Leucine Rich Repeat Kinase 1 and 2 (LRRK1 and LRRK2) are homologs in the ROCO family of proteins in humans. LRRK1 and LRRK2 have a similar domain organization: an N-terminal half containing Ankyrin (ANK) and Leucine Rich Repeats (LRR), and a catalytic C-terminal half containing the ROC–COR ROCO signature, followed by the kinase and a WD40 domain. Despite their shared domain architecture and involvement in intracellular trafficking, their disease associations are strikingly different: LRRK2 is involved in familial Parkinson’s disease while LRRK1 is linked to bone diseases. LRRK1 and LRRK2 use different mechanisms of autoinhibition, with LRRK1 having a second level of autoinhibition absent in LRRK2.

We purified LRRK1(Δ1–19), where the N-terminal 19 residues, predicted to be disordered, were deleted, and imaged it in the presence of Rab7a, ATP and GTP. Most particles classified as monomers, with a small subset forming dimers. The monomer particles yielded a 3.6-Å structure of LRRK1(Δ1–19). In contrast, the LRR of LRRK1 is shifted towards its WD40 domain, leaving its kinase’s active site exposed. The only interaction made by the LRR domain with the rest of LRRK1(Δ1–19) is a contact with the kinase’s C-lobe. The kinase domain of LRRK1 is in the open, or inactive, conformation with its DYG motif (a tripeptide involved in ATP binding) ‘out’. Even though the overall conformation of LRRK1(Δ1–19) would not prevent a Rab substrate from being engaged, we did not see any density for Rab7a in our LRRK1 map. This could be explained in part by the presence of an autoinhibitory loop extending from COR-B into the kinase active site, which we discuss below. An unusual feature of LRRK1 is the length of its kinase’s αC helix: it is approximately four turns longer than is typical in kinases. The extra residues pack against the COR-B domain through an extensive hydrophobic interaction that is unique to LRRK1.

> SAVCPERAMETLNGAGDTGGKPSTRGGDPAARSRRTEGIRAAYRRGDRGGARDLLEEACDQCASQLEKGQLLSIPAAYGDLEMVRYLLSKRLVELPTEPTDDNPAVVAAYFGHTAVVQELLESLPGPCSPQRLLNWMLALACQRGHLGVVKLLVLTHGADPESYAVRKNEFPVIVRLPLYAAIKSGNEDIAIFLLRHGAYFCSYILLDSPDPSKHLLRKYFIEASPLPSSYPGKTALRVKWSHLRLPWVDLDWLIDISCQITELDLSANCLATLPSVIPWGLINLRKLNLSDNHLGELPGVQSSDEIICSRLLEIDISSNKLSHLPPGFLHLSKLQKLTASKNCLEKLFEEENATNWIGLRKLQELDISDNKLTELPALFLHSFKSLNSLNVSRNNLKVFPDPWACPLKCCKASRNALECLPDKMAVFWKNHLKDVDFSENALKEVPLGLFQLDALMFLRLQGNQLAALPPQEKWTCRQLKTLDLSRNQLGKNEDGLKTKRIAFFTTRGRQRSGTEAASVLEFPAFLSESLEVLCLNDNHLDTVPPSVCLLKSLSELYLGNNPGLRELPPELGQLGNLWQLDTEDLTISNVPAEIQKEGPKAMLSYLRAQLRKAEKCKLMKMIIVGPPRQGKSTLLEILQTGRAPQVVHGEATIRTTKWELQRPAGSRAKVESVEFNVWDIGGPASMATVNQCFFTDKALYVVVWNLALGEEAVANLQFWLLNIEAKAPNAVVLVVGTHLDLIEAKFRVERIATLRAYVLALCRSPSGSRATGFPDITFKHLHEISCKSLEGQEGLRQLIFHVTCSMKDVGSTIGCQRLAGRLIPRSYLSLQEAVLAEQQRRSRDDDVQYLTDRQLEQLVEQTPDNDIKDYEDLQSAISFLIETGTLLHFPDTSHGLRNLYFLDPIWLSECLQRIFNIKGSRSVAKNGVIRAEDLRMLLVGTGFTQQTEEQYFQFLAKFEIALPVANDSYLLPHLLPSKPGLDTHGMRHPTANTIQRVFKMSFVPVGFWQRFIARMLISLAEMDLQLFENKKNTKSRNRKVTIYSFTGNQRNRCSTFRVKRNQTIYWQEGLLVTFDGGYLSVESSDVNWKKKKSGGMKIVCQSEVRDFSAMAFITDHVNSLIDQWFPALTATESDGTPLMEQYVPCPVCETAWAQHTDPSEKSEDVQYFDMEDCVLTAIERDFISCPRHPDLPVPLQELVPELFMTDFPARLFLENSKLEHSEDEGSVLGQGGSGTVIYRARYQGQPVAVKRFHIKKFKNFANVPADTMLRHLRATDAMKNFSEFRQEASMLHALQHPCIVALIGISIHPLCFALELAPLSSLNTVLSENARDSSFIPLGHMLTQKIAYQIASGLAYLHKKNIIFCDLKSDNILVWSLDVKEHINIKLSDYGISRQSFHEGALGVEGTPGYQAPEIRPRIVYDEKVDMFSYGMVLYELLSGQRPALGHHQLQIAKKLSKGIRPVLGQPEEVQFRRLQALMMECWDTKPEKRPLALSVVSQMKDPTFATFMYELCCGKQTAFFSSQGQEYTVVFWDGKEESRNYTVVNTEKGLMEVQRMCCPGMKVSCQLQVQRSLWTATEDQKIYIYTLKGMCPLNTPQQALDTPAVVTCFLAVPVIKKNSYLVLAGLADGLVAVFPVVRGTPKDSCSYLCSHTANRSKFSIADEDARQNPYPVKAMEVVNSGSEVWYSNGPGLLVIDCASLEICRRLEPYMAPSMVTSVVCSSEGRGEEVVWCLDDKANSLVMYHSTTYQLCARYFCGVPSPLRDMFPVRPLDTEPPAASHTANPKVPEGDSIADVSIMYSEELGTQILIHQESLTDYCSMSSYSSSPPRQAARSPSSLPSSPASSSSVPFSTDCEDSDMLHTPGAASDRSEHDLTPMDGETFSQHLQAVKILAVRDLIWVPRRGGDVIVIGLEKDSGAQRGRVIAVLKARELTPHGVLVDAAVVAKDTVVCTFENENTEWCLAVWRGWGAREFDIFYQSYEELGRLEACTRKRR>[2x]GAMGQTTFTELMQQLFLKLGLNHQVNENDV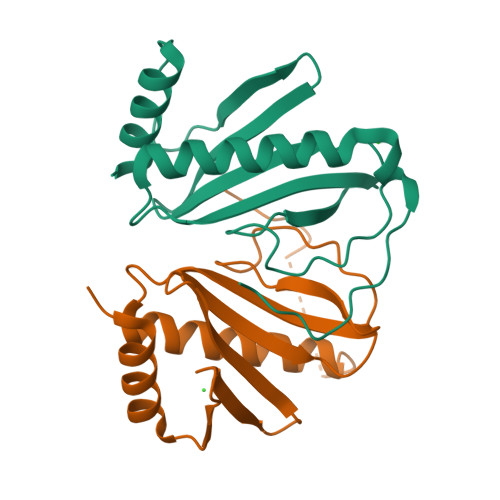YTFEVDGHIQVLIACYHQQWVQLFSELGADLPTNDNLFGEHWPAHVQGRLDGKSILWSQQSLVGLDIDEMQAWLERFIDDIEQRKEPQNTKFQPNSTSPILFI>ESPLPKPVLDTNGKELNPNSSYRIISIGRGALGGDVYLGKSPNSDAPCPDGVFRYNSDVGPSGTPVRFIPLSGGIFEDQLLNIQFNIATVKLCVSYTIWKVGNLNAYFRTMLLETGGTIGQADSSYFKIVKLSNFGYNLLYCPITPPFLCPFCRDDNFCAKVGVVIQNGKRRLALVNENPLDVLFQEV[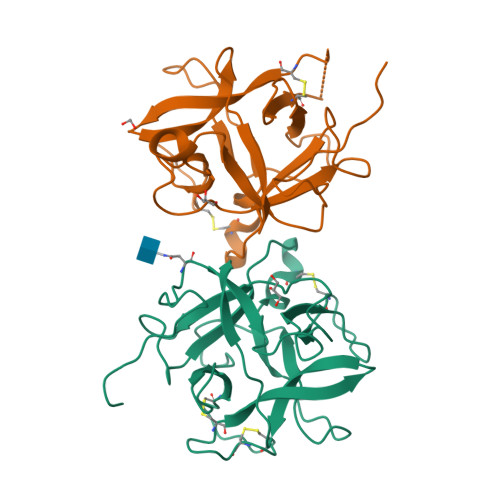2x]>MQWYLVAALLTILTSSQGILTTLSQSNGKYNYDYATIPFLAELFKLSVSGFFLWKECRTSPSVRMTKEWRSVRLYVVPSVIYLIHNNVQFATLTYVDPSTYQIMGNLKIVTTGILFRLVLKRKLSNIQWMAIVLLAVGTTTSQVKGCGDSPCDSLFSAPLEGYLLGILSACLSALAGVYTEYLMKKNNDSLYWQNVQLYTFGVIFNMGWLIYGDFKAGFELGPWWQRLFNGYSITTWMVVFNLGSTGLLVSWLMKYSDNIVKVYSTSMAMLL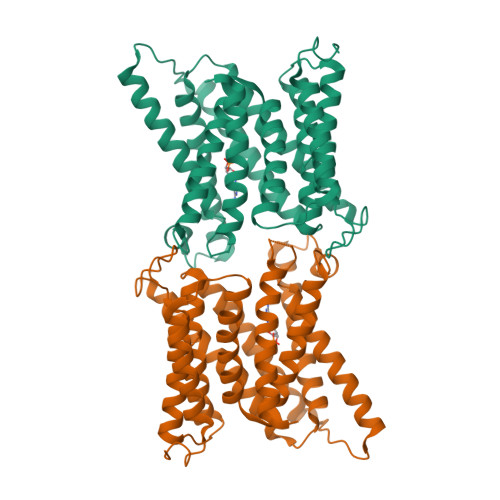TMVLSIYLFSVKATIQLFLGIIICIISLQMYFMPVHMLIELPQTLPVTSK[2x]>GSTGSVYGRQAIEYVIKRMGSQMGVPYSWGGGSLDGPSKGVGDGANITGFDCSGLMRYGFAGVGVLIPRFSGDQYNAG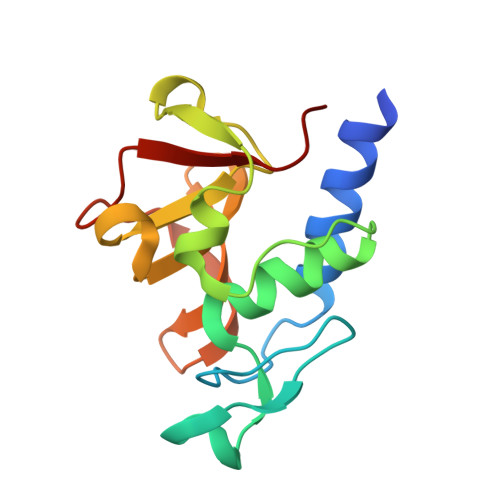RHIPQDQARRGDLIFYGPGGSQHVTMYLGNGQMLEASGSAGKVTVSPVRKPGMTPFLTRIIEY[2x]>[8x]GSGSPLA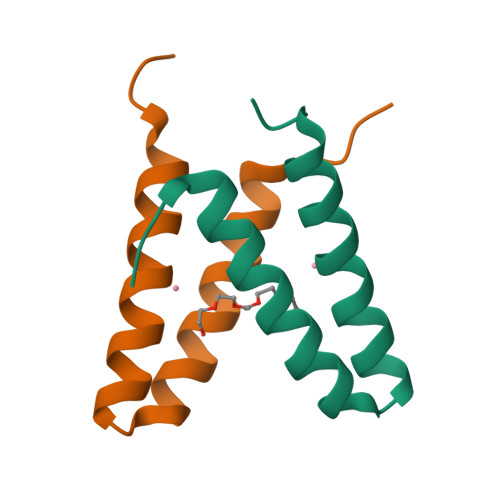QQIKNIHSFIHQAKAAGRMDEVRTLQENLHQLMHEYFQQSD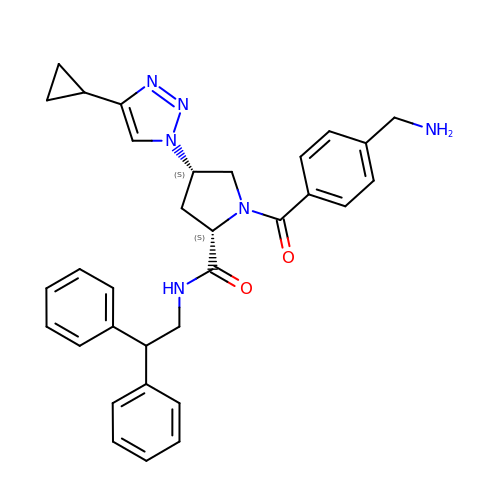(2~{S},4~{S})-1-[4-(aminomethyl)phenyl]carbonyl-4-(4-cyclopropyl-1,2,3-triazol-1-yl)-~{N}-(2,2-diphenylethyl)pyrrolidine-2-carboxamide | C32 H34 N6 O2 | YBZBHUMSHGXQNF-FIBWVYCGSA-N>[4x]MAQQSTKNETALLVAKSAKSALQDFNHDYSKSWTFGDKWDNSNTMFETFVNKYLFPKINETLLIDIALGNRFNWLAKEQDFIGQYSEEYVIMDTVPINMDLSKNEELMLKRNYPRMATKLYGNGI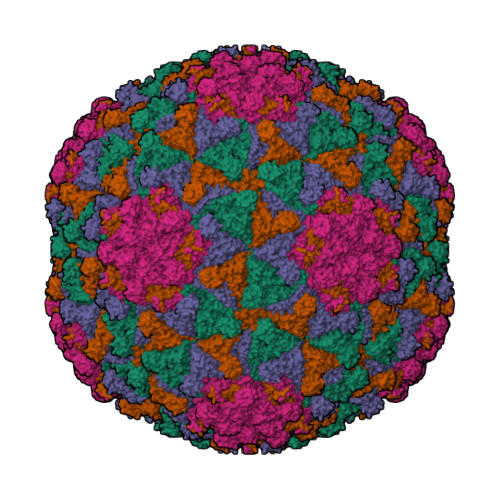VKKQKFTLNNNDTRFNFQTLADATNYALGVYKKKISDINVLEEKEMRAMLVDYSLNQLSETNVRKATSKEDLASKVFEAILNLQNNSAKYNEVHRASGGAIGQYTTVSKLKDIVILTTDSLKSYLLDTKIANTFQIAGIDFTDHVISFDDLGGVFKVTKEFKLQNQDSIDFLRAYGDYQSQLGDTIPVGAVFTYDVSKLKEFTGNVEEIKPKSDLYAFILDINSIKYKRYTKGMLKPPFHNPEFDEVTHWIHYYSFKAISPFFNKILITDQDVNPKPEEELQE;>MYEGNNMRSMMGTSYEDSRLNKRTELNENMSIDTNKSEDSYGVQIHSLSKQSFTGDVEEE[4x]>[2x]MSHHHHHHKGLYFQQSSTDEEITFVFQEKEDLPVTEDNFVKLQVKACALSQINTKLLAEMKMKKDLFPVGREI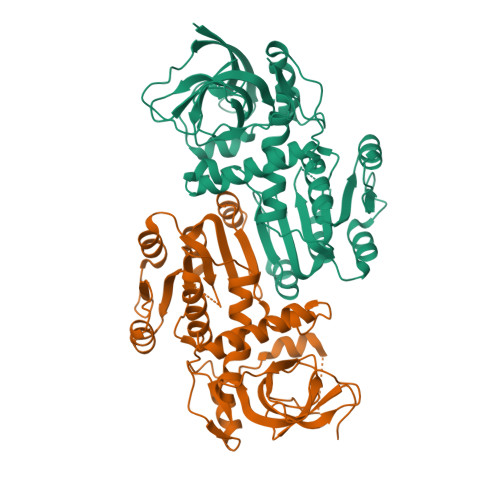AGIVLDVGSKVSFFQPDDEVVGILPLDSEDPGLCEVVRVHEHYLVHKPEKVTWTEAAGSIRDGVRAYTALHYLSHLSPGKSVLIMDGASAFGTIAIQLAHHRGAKVISTACSLEDKQCLERFRPPIARVIDVSNGKVHVAESCLEETGGLGVDIVLDAGVRLYSKDDEPAVKLQLLPHKHDIITLLGVGGHWVTTEENLQLDPPDSHCLFLKGATLAFLNDEVWNLSNVQQGKYLCILKDVMEKLSTGVFRPQLDEPIPLYEAKVSMEAVQKNQGRKKQVVQF2-AMINO-8-METHYLQUINAZOLIN-4(3H)-ONE | C9 H9 N3 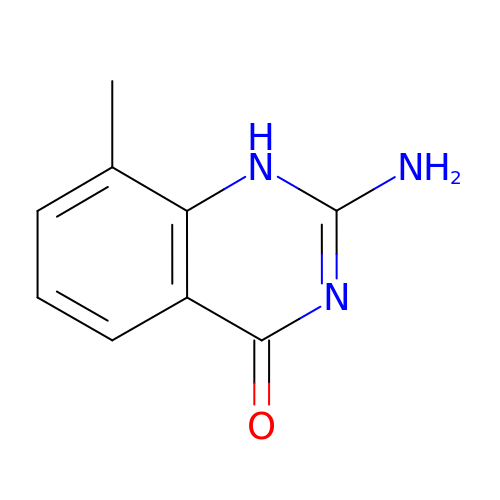O | NLLZAHIPYDRNRQ-UHFFFAOYSA-N>GQDMVSPPPPIADEPLTVNTGIYLIQCYSLDDKAETFKVNAFLSLSWKDRRLAFDPVRSGVRVKTYEPEAIWIP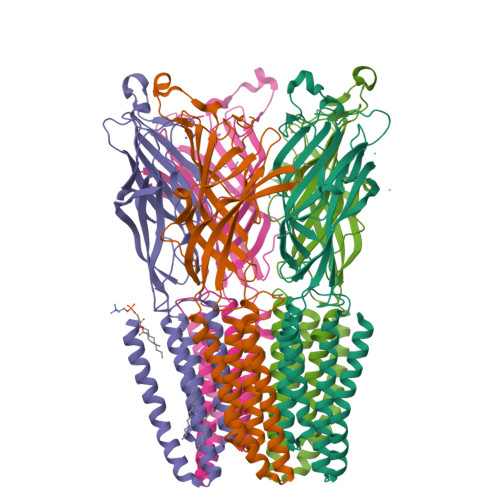EIRFVNVENARDADVVDISVSPDGTVQYLERFSARVLSPLDFRRYPFDSQTLHIYLIVRSVDTRNIVLAVDLEKVGKNDDVFLTGWDIESFTAVVKPANFALEDRLESKLDYQLRISRQYFSYIPNIILPMLFILFISWTAFWSTSYEANVTLVVSTLIAHIAFNILVETNLPKTPYMTYTGAIIFMIYLFYFVAVIEVTVQHYLKVESQPARAASITRASRIAFPVVFLLANIILAFLFFGF[5x]> MRLLKYPLDIHNEQVNALAALGPYIILAGSGGHVMAWRQQQLVDTAFDRVMIKDLKPEVSFQVDQDTTGDIFFITGDLETLYIGSEHRLWGYSGWLCRDTNNINSVEKMNSKLLFECKSPSTITDVKYDINLGILFVLLSNENKILLFRHKTFDKLSEITIDKASKPITGIIDPTGQTFTVMTSDRSILVYQINKTGTHKLINKLTQHVQMYPLHYRISMSPQADILPVINSVKGVPNNATSCTALLDRNNNYKVTKTLVTPSSNGCRVLVYSPAFYEKPNLKKGTSTRYNLIATSGSTDGTILVWNTKRMKPLFNALQVSSTAINDMSWSQDGFTLFAISNDATLYTFAFQEKDLGVALPQTEIKSLQEVNKKLPKLEEPLAEQIPKSFPENIKLEESASAAPIPNDIGRSAVGKKPTKKKTANNQTNGIKTIQSTSMEFNTPSYTVPRDLKRKPKEATPSNIAPGSKKQKKELQPIDFLDTGLLLPNTSFSRIRLATPKIRSTFKYSPINNPNLILDVKNGSGNEQRPTIVKLTSKVLDQDQVLFQDFIPKLITICTAGDTFWSFCSEDGSIYIYSDSGRKLMAPLVLGVSISFLEACGTYLLCLTSIGELYCWNIEQKKLAFPTNTIYPLLNPSLRYSDDILTRAENITLCSITKKGVPLVTLSNGDGYLFDKNMETWLLVSDGWWAYGSQYWDTTNTTGLSSSKANTDSFNGSESNINEIVSDIKNDNQSIINFLECKTNDELNRKGRIKNLQRFARTILMKEGFENMEEIVTLSHLENKILISIRLEEPEEFSKLMMVYCIRLSELGYMDRLNDVFQWLYDDLPISGTGSAFADKDFKRNLLKKILIACGDIRQVQRVTTRYAKEMNIIS;> MSMFNALNSNIEGEQYEAEEHSRELQIEQSFNILQDALIDLKNKDFEKSDSKFQELFQIDVVKPDRWGMYRNSSPTLDNLRYLCYRNRGMYYHLYLENNYERLNSQELVNCILKAVENLVESIQHSDADFAVTDLLARIFKSFNSVKLERLISEYEFTKQENLSLLLGRHRKFLLNDLTLMMNNYVELTNKLLVPNLSDNTIFERYHLEKYKDIKPEPLAFGPILSRISEMKKQDEEIMKKLDVFNVTLNEESWDEVAKALKNLLPSVKTSSLIGRNMDPYNEIEEPIEAVKFELSEAINNTPSLDRESERQEEEQDNESVRADDKSGNLAPSDIQTNEEARPNKRTDEHIDSTKPLQRSSKRFKEREQENSKELVMDVHKRFFGEFNTLLSYIHILPFCDFDTFASKFIIGSSDKQPEKFIPYTDLYECLKSWSSRYTDIFNQNDYLSSGSNENEELFQLNALLKSNAFDDKESFPRYLNDLDSDHIRSFISEVNAGNLHFHQVRLKLLFKLLGTYDEGNGRRLIIDYLWESQLLKIVLWFVFGIESNIFALINKNKRQCKYLALSIYELLVNHLGNIVEEITNKRIQGHKSADLKSQRNKVEKRIRSWHTLLEQIADEKDKELYVHFQWTHYCFLQYTCDIVDSRLSETLTSLENTIKDSDSSLDIAYPNYRHIPALNLNTVQSQKRKIRIIQNITVEDISEDTNSDTHSENHLETLEKVLLHILHPSTNHSNIDEEMVSFIFNSPFLLKIRLWGVLFSSYVKKSSIQDVQRIYFHVLDFMKGALTSPVYKESNPHGRHQMLLTVLTAIGYLSSQLTAILNSNRWESSDFVLEDYMFEKLLQTFFFFYTVLFYESSAVNDVSNKSFFKRASKSSGKMKDIMIDLATLILYYYDLQAKLRTPAEQGIETTELIWSLHTLFGHFHFCDASNGKFLDLAEKLLCQFINNDSFLQLKQILWCRYHYAIASDNFSPDLHDTKAVEMEKIHSLPLGTYLIKLQYQNKNPYLSSSKTTLKQIMDNIIEKIGDPSTLDNHIISRNSFLLNEYLSRPITADLLKHTFSGATSLYLTSPNDELQQGMTAGLFYVSSLQSLGLYKMRKKSMQARPSELDSIIRMLKNDIIYNTNRFESWILLGKCYSYIVEDDLIWTSDKITVPEKKDVIALTQRKAILCYLMAISIYYSKLDRTIDDKKIILEALDDLGSMLISGYYNPMNKLCFSWKSSAENTMRLSETGEVVMEKTKKITTISDFNIEQSIFLCFNRACSLSGDIKSQDDVFVLNWSSFYNLAKFFFKTDGGNNCKLVAKYITQGCQIAYESSPAKDPIIEPHYLLVNACYKWVKRGVIGVNEALTLLSKDNQFFQEQEEFWVNDEGLAWDYQEKFFFDKIIRLLRHLLSVDKKKWQHRPRYRIARILFDDLGDVNGALEEMDSLISAKSINKNLVNIWKPDFERPGKHFIYTYQYLVLYLDLLFAIKDFNTTGLVIKKLRRFGSGTVNVNELLERAINVYTQSAKIKLQLQDKSYVEQILPTLNYQEFLKISEQLNQVFDQGKYPEEISSGLKLAFQLKKGHSGIAFDSVCLGIYFEYLYFPLARQDQSLTDVNDENNPALPSSGSVTSKSTPDPT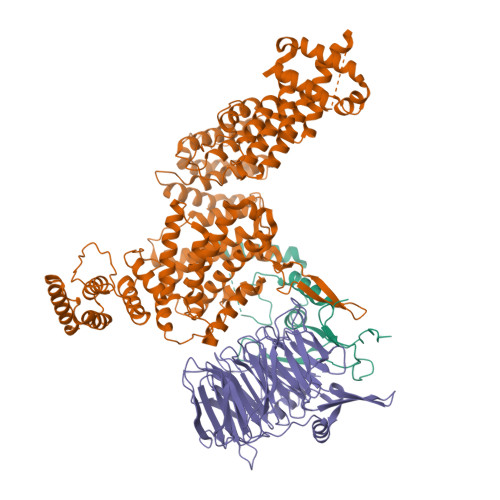SKPSAIKKRVTKKEVFDRVRLLVDKIT;> MDQKAIVLDNSKSGSKQTKSSGKMQTQTDTNAEVLNTDNSIKKETGSDSEDLFNKFSNKKTNRKIPNIAEELAKNRNYVKGASPSPIIISGSSSTSPSGPSSSSTNPMGIPTNRFNKNTVELYQHSPSPVMTTNKTDTEEKRQNNRNMDNKNTPERGSSSFAAKQLKISSLLTISSNEDSKTLHINDTNGNKNSNAASNNIPSAYAELHTEGNSIESLIKPPSSPRNKSLTPKVILPTQNMDGTIAKDPHLGDNTPGILIAKTSSPVNLDVESTAQSLGKFNKSTNSLKAALTKAPAEKVSLKRSISSVTNSDSNISSSKKPTSEKAKKSSSASAILPKPTTTKTSKKAASNSSDSTRKKNASNKTTSAIKKESNAGSKLNTVKKENSSLSSIKATEKEKDKGGNSTEAKNSTSNVRKEPTAKSPKRLVAAPTVSPPKILQTAETKAKEPSILIDVPLYQADTNDYLDENGQVIFNLSTLIKEKYHPKSKELAQLKDSKRNLLMQLSDHSNGSLEKEKDEEGDVIELDDDEDMEEDEGEIDTETNTVTTTISPKKKSHPMKGKNLIGKYDVEDPFIDDSELLWEEQRAATKDGFFVYFGPLIEKGHYASLERANGTMKRGGVKNK4-[4-[[5-fluoranyl-4-[[3-(propanoylamino)phenyl]amino]pyrimidin-2-yl]amino]phenoxy]-~{N}-methyl-pyridine-2-carboxamide | C26 H24 F N7 O3 | 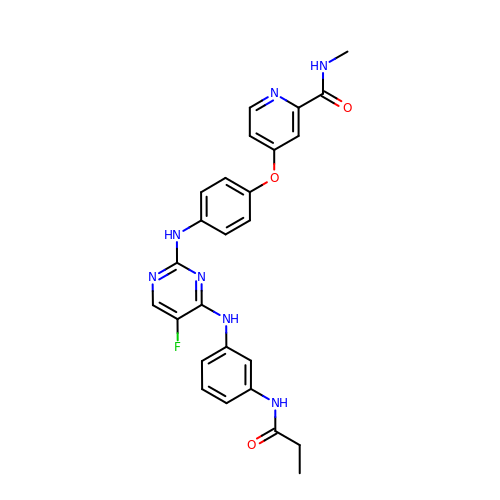JTYHXYSMSXOMLI-UHFFFAOYSA-N> MFENITTAPADPILGLADLLRADERPGKIDLGMGVYNDETGKTPVLTSVKKAEQYLLENETTKNYLGIDGIPEFGRCTQELLFGKGSALINDKRARTAQTPGGTGALRVAADFLAKNTSVKRVWVSNPSWPNHKSVFNSAGLEVREYAYYDAENHTLDFDALINSLNEAQAGDVV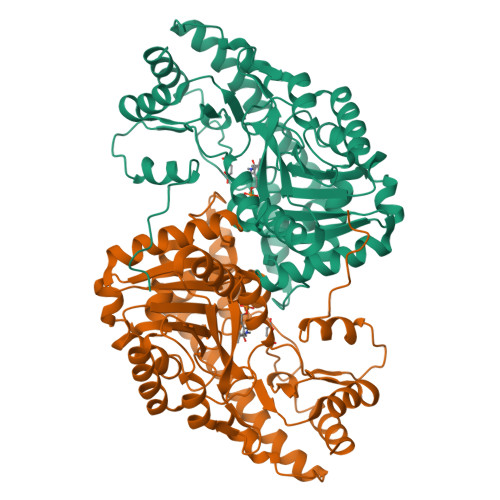LFHGCCHNPTGIDPTLEQWQTLAQLSVEKGWLPLFDFAYQGFARGLEEDAEGLRAFAAMHKELIVASSYSKNFGLYNERVGACTLVAADSETVDRAFSQMKAAIRVNYSSPPAHGASVVATILSNDALRAIWEQELTDMRQRIQRMRQLFVNTLQEKGANRDFSFIIKQNGMFSFSGLTKEQVLRLREEFGVYAVASGRVNVAGMTPDNMAPLCEAIVAVL4-(1,2,3-thiadiazol-4-yl)phenyl ethylcarbamate | C11 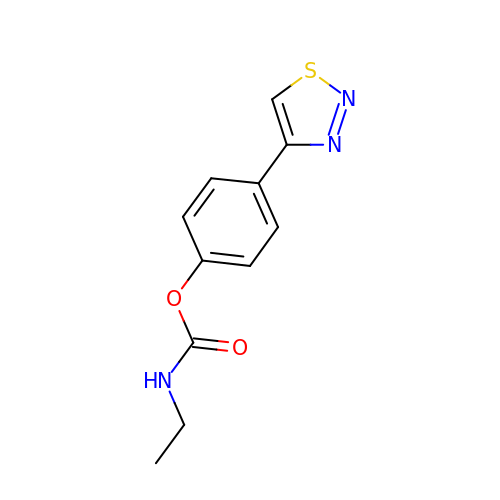H11 N3 O2 S | VSHNRASUUBQGMG-UHFFFAOYSA-N>[2x]MPNIKIFSGSSHQDLSQKIADRLGLELGKVVTKKFSNQETCVEIGESVRGEDVYIVQSGCGEINNNLMELLIMINACKIASASRVTAVIPCFPYARQDKKDKSRAPISAKLVANMLSVAGADHIITMDLHASQIQGFFDIPVDNLYAEPAVLKWIRENISEWRNCTIVSPDAGGAKRVTSIADRLNVDFALIHKERKKANEVDRMVLVGDVKDRVAILVDDMADTCGTICHAADKLLSAGATRVYAILTHGIFSGPAISRINNACFEAVVVTNTIPQEDKMKHCSKIQVIDISMILAEAIRRTHNGESVSYLFSHVPLLEHHHHHH

PRPP is formed from ATP and D-ribose-5-phosphate (R5P) by the phosphoribosyl pyrophosphate synthetases (PRSs). The human PRS family, which has 3 isoforms (hPRS1, hPRS2 and hPRS3), belongs to the class I PRSs that requires divalent metal ions such as Mg2+ as the activator, inorganic phosphate ion for activity, and ATP or dATP as the diphosphoryl donor. Due to the important role of PRPP in the nucleotide metabolic process, the stability of PRPP content is essential for cell physiology and is predominantly controlled by hPRS1, the ubiquitously expressed human PRPP synthetase. Mutations in hPRS1 affect vital cell functions and are related to many diseases and disorders.

We determined the crystal structures of the E43T, D65N, A87T, M115T and Q133P mutations at a resolution of 3.0 Å, 2.14 Å, 3.3 Å, 2.11 Å and 2.74 Å, respectively, with 2 molecules in each asymmetric unit. Overall, the structures of all the five structures are highly similar to that of the wild type PRS1 with RMSD listed in S2 Table. In the D65N structure, the salt bridge between Asp65 and Lys34 in the PRS1 structure is replaced by a hydrogen bond between Asn65 and Lys34, which might reduce the restraint of the ATP binding motif β2–3. In order to confirm this, we performed the MD simulation, which indicates that there are fewer contacts between the Gln65 in D65N mutant and the ATP binding motif β2–3. The low activity D65N mutation affects the ATP-binding β2–3 strands directly.> GENLLLPDLWLDFLQLSPIFQRKLAAVIACVRRLRTQATVYPEEDMCMAWARFCDPSDIKVVILGQDPYHGGQANGLAFS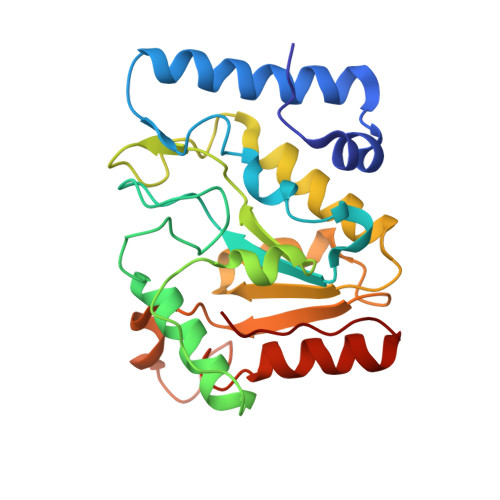VAYGFPVPPSLRNIYAELHRSLPEFSPPDHGCLDAWASQGVLLLNTILTVQKGKPGSHADIGWAWFTDHVISLLSERLKACVFMLWGAKAGDKASLINSKKHLVLTSQHPSPLAQNSTRKSAQQKFLGNNHFVLANNFLREKGLGEIDWRL> MHHHHHHHHHHSGQNLYFQGHMATFISVQLKKTSEVDLAKPLVKFIQQTYPSGGEEQAQYCRAAEELSKLRRAAVGRPLDKHEGALETLLRYYDQICSIEPKFPFSENQICLTFTWKDAFDKGSLFGGSVKLALASLGYEKSCVLFNCAALASQIAAEQNLDNDEGLKIAAKHYQFASGAFLHIKETVLSALSREPTVDISPDTVGTLSLIMLAQAQEVFFLKATRDKMKDAIIAKLANQAADYFGDAFKQCQYKDTLPKEVFPVLAAKHCIMQANAEYHQSILAKQQKKFGEEIARLQHAAELIKTVASRYDEYVNVKDFSDKINRALAAAKKDNDFIYHDRVPDLKDLDPIGKATL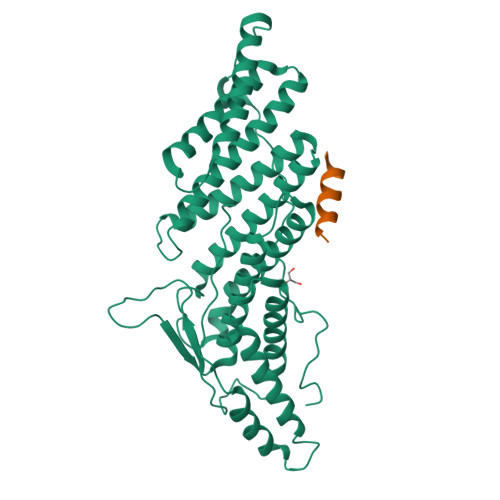VKSTPVNVPISQKFTDLFEKMV;> EDDDIKQLAAWAT The Ser/Thr protein kinase Tor is a hub for cellular homeostatic regulation. While some yeast species such as Saccharomyces cerevisiae have two genes that encode Tor1 and Tor2 proteins, mammalian cells have a single gene encoding mTOR910. Both Tor and mTOR occur in two complexes known as TORC1 and TORC2. Lst8 is a requisite component for both TORC1 and TORC2. PIKKs share a catalytic core consisting of a kinase domain flanked by a helical FAT domain (named after FKBP12 Rapamycin Associated Protein (FRAP)–ATM–TRRAP) at the N-terminus and a short FAT-C domain at its C-terminus36.

Focusing on the heterodimer that forms the core of both TORC1 and TORC2, we have determined a 6 Å resolution structure of the full-length Tor–Lst8 complex from the thermotolerant yeast Kluyveromyces marxianus (KmTor). Our structure shows that KmTor–Lst8 forms a dimer of heterodimers, in which the two KmTor subunits embrace each other with their helical solenoids. The Fourier shell correlation plot suggests that the overall resolution of the structure is ∼6 Å, with the highest local resolution (5 Å) corresponding to the FATKIN and the N- and C-terminal regions of the α-solenoid that contact the FATKIN. The structure of each monomer shows an extensive N-terminal helical solenoid with a complex topology that precedes the FATKIN. The N-terminus of KmTor forms a highly curved spiral consisting of about 800 residues arranged into 36 helices (residues 64–837). The spiral is followed by a linker (residues 838–894) that runs along the surface of the FATKIN to connect the spiral to a region that we will refer to as the 'bridge' (residues 895–1169). The bridge is followed by a 32-residue linker that we refer to as the ‘railing' (residues 1170–1201) that folds back and runs over the entire length of the bridge, ending in several helices (Nα52–Nα56) that form a 'cap' (residues 1202–1292), which packs between the N-terminal end of the bridge and the TRD1 of the FATKIN. The largest interface between the two KmTor subunits occurs at the periphery of the dimer and involves a region of the spiral (helices Nα25, Nα27 and Nα29) of one molecule contacting the bridge (helices N\α44, N\α46, N\α48 and N\α50) of the other molecule. The second, smaller interface consists of the HRD domain of one Tor interacting with the HRD of the other, via three helices (α24, α26 and α28) making intermolecular contacts at the center of the dimer. This dimeric arrangement of KmTor places the two active sites facing away from each other, with the two FATKINs resting on a cradle made up of two N-terminal helical solenoids.

>[2x]ELLEGELKTAALAQHDEAMGGSLRRKGESVKKRLVSGTAASLQELSLQPSSNGIASAGKSEDGEAGDGMSGEFGAALTDSNVENNVKAFDLIFTKLKSTNQLERVAASYELKSCLISLAREVSTEYFQRFSNDINNKVFELIHGTDSNEKLGGVLAVDTLIDFYSHTDELPNQTSRLANYLRVLIPSNDIEVMRAAATTLGKLAVPGGTLTSEFVEFEVKTCIEWLTTSPESSSSNSKQEYRKHASLLIISSIAHNSPYLLYPFVNSILDNIWRALRDTKLVIRTDAAVTLGKCLTIINDRDSSLTKKWVQRLFNGCIYGLQLNTTVSIHGTLLVYRQLVSLEGGYLKDKYEEIYETTMKHRDNKNIIIRKEIYAIIPVLAAFDPKLFTQKYLDATMIHYLTLLKNMTSHQIALSDKGPILVSIGDIAYHVGSEIGPYLDAIVENLRDGLETKFKTRKEFEKDIFYCVSKLACAVRPLLAKYLNRGLLDALLACPLSDHMQETLLVICEKIPSMEVTVNEKLLNIICLVLSGEKFRPPGSPTPMKSLSSETARAYRDQSLLRKTGENNNDTLDAMILRKALRMLSDIKPKYSLTEFIRRVIISYMEHDNMQVRKLAALTSCDLFVKDSICKQTSLYALNVVSEVLSKLLTVAITDPVAEIRLEILKHLDRNFDPQLSQPDNTKLLFMALNDEVFAIQMEAMKICGRLALVNPAYVIPSLRKTLIQLLTELKHSKMTRKKEECASLLCTLISSSSDVTKPYLEPVIEILLPKSQDPSSAVASTALKALGEISVVGGEDMLPFLDELMPLIIDTFQDQSNSFKRGAALKALGQLAASSGYVIDPLLDYPELLGVLINILKSESSQNIRRETVRLIGILGALDPYKHREVERTSITNITSEQNAPPIDVALLMQGMSPSNEEYYPTVVIGVLMKILKDPSLSIHHSTVIQAIMHIFQTMGLRCVIFLKQIIPGFILVMHTCPPSLLELYFQQLSVLISIVKQHIRPHVTEIVDVISEFFPVLKLQLTIISVIESLSRALEGEFNPHLPTILSLFLDVLEKDQSNKKVVSVRILKSLVVFGPHLEEYVHLVLPTIIKLSEFSSGNLKKAAIITIGRLSKNVNALEMSSRIVQALVRVLNTSETEYVKATMNTLSLLLLQLNIDFTVFIPVINKTLVKQNIQHTIYDRLVAKLLNNEPLPTKIIIDKDFDLPNKEMDDVKVASKKLPVNQMVLKNAWDCSQQRTKEDWQEWIRRLSISLLKESSSHALRACSGLAGIYYPLARELFNASFASCWGELYTQYQEDLIQSLCAALSSPNNPPEIHQTLLNLVEFMEHDDKPLPISISTLGEYAQRCHAYAKALHYKELEFIEEPSTSTIESLITINNQLHQTDAAIGILKHAQQHHDLQLKETWYEKLQRWDDALNAYNKREAAGEDSVEVTIGKMRSLHALGEWDQLSELAADKWASSQLEVKRAIAPLAAGAAWGLAQWDRVEQYIEVMKPQSPDKAFFDAILCLHRNNFEKAAEHIFSARDLLVTEMSALVNESYNRAYGVVVRTQMVAELEEIIQYKKLPQGSERRAMIRKTWNKRLLGCQKNVDVWQRVLKVRSLVIKPKQDMKVWIKFANLCRKSGRLGLAQKTLNTLLEESGDPKNPNTARAPPPVVYAQLKYMWATGSQKEALNHLISFTSRMAHDLGLDPSNMIAQSVPQNSSVSQHHIEDYTKLLARCFLKQGEWRVSLQPNWRLENPDAILGSYLLATHFDKTWYKAWHNWALANFEVTSSLTQRIKDDKVPPTLEDASTEFTNGAVAGLNANDNFPPELVQRHVVPAIKGFFHSIALSQSSSLQDTLRLLTLWFKFGGIPEAAQAMHEGFGLIKIDNWLEVIPQLISRIHQPNQTVSRSLLSLLADLGKAHPQALVYPLTVAIKSDSVSRQRAALSIIDKMRMHSPKLVNQAELVSDELIRVAVLWHELWYEGLEDASRQFFGEHNTEKMFATLEPLHEMLKRGPETLREISFQNSFGRDLNDAYEWVLNYKRTKDINNLNQAWDIYYNVFRRISRKLPQLQTLDLQHVSPKLSAAKDLELAVPGTYHAGKPIVRITHFEPVFTVISSKQRPRRVIIKGSDGKDYQYLLKSHEDIRQDNLVMQLFGLVNTLLQNDPESFQRHLNIQQYPAIPLSPKTGLLGWVPNSDTFHVLIREHREASKIPLNIEHRIMLQMAPDYDNLTLLQKVEVFTYALDNTKGQDLYKVLWLKSRSSESWLDRRTTYTRSLAVMSMVGYILGLGDRHPSNLMLDRITGKVVHIDFGDCFEAAILREKYPEKVPFRLTRMLTYAMEVSGIEGSFRITCENVMMVLRDNKESLMAILEAFAYDPLINWGFDLPTHAVMEQTGIDLPLANPSELLRKGVISVEDAAKMELQQKAEVRNARATLVLKRIADKLTGNDFPRCQELSVPDQVDKLIQQATSVENLCQHYIGWCSFW;>[2x]MSVILASAGYDHTIRFWEALTGVCSRTIQHADSQVNRLEITSDKKYLAAAGHLHVRLYDIRSNNPNPVSSFEGHKGNVTSIAFQQENRWMVSSSEDGTIKVWDVRSPSVQRNYKHNAPVNEVAIHPNQGELISCDQDGNIRIWDLGENQCTNQLTPEDNTPLQSLSVASDGSMLVAGNNKGNCYVWRMPHHTDASTLEPVTKFKSHTKYITRVLLSADVKNLATCSADHTARVWNIEDNYQLETTLDGHQRWVWDCAFSADSAYLVTACSDHYVRLWDLSTSEIVRQYGGHHKGAVCVALNDV>[3x]SKPQPIAAANWKSGSPDSLSELIDLFNSTSINHDVQCVVASTFVHLAMTKERLSHPKFVIAAQNAGNADALASLKDFGVNWIVLGHSERRWYYGETNEIVA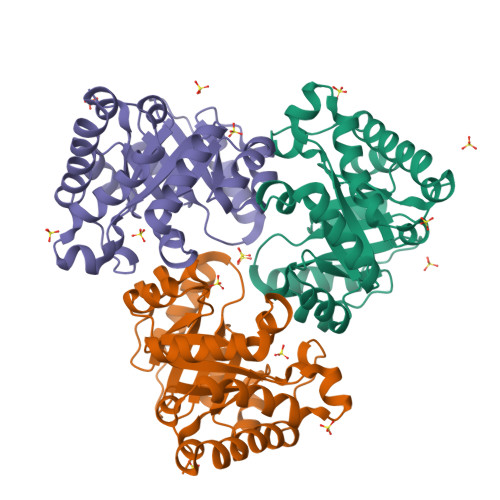DKVAAAVASGFMVIACIGETLQERESGRTAVVVLTQIAAIAKKLKKADWAKVVIAYEPVWAIGTGKVATPQQAQEAHALIRSWVSSKIGADVAGELRILYGGSVNGKNARTLYQQRDVNGFLVGLKPEFVDIIKATQ> SAKAVDYETEVVLGNGERKKIGEIVERAIEEAEKNGKLGRVDDGFYAPIDIEVYSLDLETLKVRKARANIAWKRTAPKKMMLVKTRGGKRIRVTPTHPFFVLEEGKVAMRKARDLEEGNKIATIEGLSVSWDEVAEILEYEPKDPWVYDLQVPGYHNFLANGIFVHAA

Protein splicing is catalyzed by intervening protein sequences termed inteins. As the first step toward understanding the spread and evolution of inteins and cross-talks within the “inteinome”, we determined the crystal structures of mini-inteins inserted at the same insertion site within the putative cell division control protein 21 (Cdc21) from the hyperthermophilic archaea, Pyrococcus abyssi and Pyrococcus horikoshii OT3. The cell division control protein 21 (Cdc21), belonging to the MCM (mini-chromosome maintenance) protein family, is one of the proteins invaded by several inteins. The structure of the PabCDC21-1 intein revealed the HINT fold characteristic for inteins from thermophilic organisms.

The PabCDC21-1 intein is inserted at the presumable P-loop ATP/GTP-binding motif; while, the PabCDC21-2 intein locates 27 residues downstream of the PabCDC21-1 intein insertion site. Indeed, we could obtain diffracting crystals of a variant of the PabCDC21-1 intein carrying mutations at the N- and C-terminal catalytic residues (C1A, and N164A) together with three N- and one C-extein residue (Ser-Ala-Lys and Ala, respectively). We solved the three-dimensional structure of PabCDC21-1 intein at 1.60-Å resolution by molecular replacement. The presence of N- and C-extein residues due to the active site mutations allowed us to analyze the conformation of the PabCDC21-1 intein by measuring the distance between the N-scissile peptide and the side chain of the +1 residue (Cα atom of Ala). A large distance of about 8 Å suggests an open conformation as it has been observed in most intein structures containing extein residues. PabCDC21-1 has an improved C2-symmetry interface with the loop regions at the C35 and N35 sites with hydrophobic residues L53, L58, and V60 for the N-terminal, and I121, L124, and V126 for the C-terminal subdomain (the C35 and N35 numbering for the split sites is based on the NpuDnaE intein as described in Aranko et al. (2014a) for convenience). The structure of the PabCDC21-1 intein revealed extensive hydrophobic interactions between the C2-symmetry-related N35 and C35 loops, increasing the subdomain interactions at the elevated temperature optimal for the growth of Pyrococcus abyssi. The crystal structures of the PabCDC21-1 and PhoCDC21-1 inteins showed that both mini-inteins do not have large flexible loop insertions at the HEN insertion site, unlike the MjaTFIIB intein.>[2x]MSQEQGKIYIVEDDMTIVSLLKDHLSA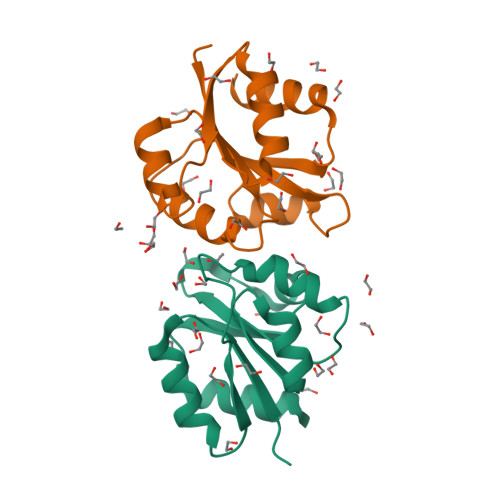SYHVSSVSNFRDVKQEIIAFQPDLILMDITLPYFNGFYWTAELRKFLTIPIIFISSSNDEMDMVMALNMGGDDFISKPFSLAVLDAKLTAILRRSQQFIQQELTFGGFTLTREGLLSSQDKEVILSPTENKILSILLMHPKQVVSKESLLEKLWENDSFIDQNTLNVNMTRLRKKIVPIGFDYIHTVRGVGYLLQDPNSSSVDKLAAALEHHHHHH>[2x]MDYKDDDDKHMSLVLNDLLICCRQLEHDRATERKKEVEKFKRLIRDPETIKHLDRHSDSKQGKYLNWDAVFRFLQKYIQKETECLRIAKPNVSASTQASRQKKMQEISSLVKYFIKCANRRAPRLKCQELLNYIMDTVKDSSNGAIYGADCSNILLKDILSVRKYWCEISQQQWLELFSVYFRLYLKPSQDVHRVLVARIIHAVTKGCCSQTDGLNSKFLDFFSKAIQCARQEKSSSGLNHILAALTIFLKTLAVNFRIRVCELGDEILPTLLYIWTQHRLNDSLKEVIIELFQLQIYIHHPKGAKTQEKGAYESTKWRSILYNLYDLLVNEISHIGSRGKYSSGFRNIAVKENLIELMADICHQVFNEDTRSLEISQSYTTTQRESSDYSVPCKRKKIELGWEVIKDHLQKSQNDFDLVPWLQIATQLISKYPASLPNCELSPLLMILSQLLPQQRHGERTPYVLRCLTEVALCQDKRSNLESSQKSDLLKLWNKIWCITFRGISSEQIQAENFGLLGAIIQGSLVEVDREFWKLFTGSACRPSCPAVCCLTLALTTSIVPGTVKMGIEQNMCEVNRSFSLKESIMKWLLFYQLEGDLENSTEVPPILHSNFPHLVLEKILVSLTMKNCKAAMNFFQSVPECEHHQKDKEELSFSEVEELFLQTTFDKMDFLTIVRECGIEKHQSSIGFSVHQNLKESLDRCLLGLSEQLLNNYSSEITNSETLVRCSRLLVGVLGCYCYMGVIAEEEAYKSELFQKAKSLMQCAGESITLFKNKTNEEFRIGSLRNMMQLCTRCLSNCTKKSPNKIASGFFLRLLTSKLMNDIADICKSLASFIKKPFDRGEVESMEDDTNGNLMEVEDQSSMNLFNDYPDSSVSDANEPGESQSTIGAINPLAEEYLSKQDLLFLDMLKFLCLCVTTAQTNTVSFRAADIRRKLLMLIDSSTLEPTKSLHLHMYLMLLKELPGEEYPLPMEDVLELLKPLSNVCSLYRRDQDVCKTILNHVLHVVKNLGQSNMDSENTRDAQGQFLTVIGAFWHLTKERKYIFSVRMALVNCLKTLLEADPYSKWAILNVMGKDFPVNEVFTQFLADNHHQVRMLAAESINRLFQDTKGDSSRLLKALPLKLQQTAFENAYLKAQEGMREMSHSAENPETLDEIYNRKSVLLTLIAVVLSCSPICEKQALFALCKSVKENGLEPHLVKKVLEKVSETFGYRRLEDFMASHLDYLVLEWLNLQDTEYNLSSFPFILLNYTNIEDFYRSCYKVLIPHLVIRSHFDEVKSIANQIQEDWKSLLTDCFPKILVNILPYFAYEGTRDSGMAQQRETATKVYDMLKSENLLGKQIDHLFISNLPEIVVELLMTLHEPANSSASQSTDLCDFSGDLDPAPNPPHFPSHVIKATFAYISNCHKTKLKSILEILSKSPDSYQKILLAICEQAAETNNVYKKHRILKIYHLFVSLLLKDIKSGLGGAWAFVLRDVIYTLIHYINQRPSCIMDVSLRSFSLCCDLLSQVCQTAVTYCKDALENHLHVIVGTLIPLVYEQVEVQKQVLDLLKYLVIDNKDNENLYITIKLLDPFPDHVVFKDLRITQQKIKYSRGPFSLLEEINHFLSVSVYDALPLTRLEGLKDLRRQLELHKDQMVDIMRASQDNPQDGIMVKLVVNLLQLSKMAINHTGEKEVLEAVGSCLGEVGPIDFSTIAIQHSKDASYTKALKLFEDKELQWTFIMLTYLNNTLVEDCVKVRSAAVTCLKNILATKTGHSFWEIYKMTTDPMLAYLQPFRTSRKKFLEVPRFDKENPFEGLDDINLWIPLSENHDIWIKTLTCAFLDSGGTKCEILQLLKPMCEVKTDFCQTVLPYLIHDILLQDTNESWRNLLSTHVQGFFTSCLRHFSQTSRSTTPANLDSESEHFFRCCLDKKSQRTMLAVVDYMRRQKRPSSGTIFNDAFWLDLNYLEVAKVAQSCAAHFTALLYAEIYADKKSM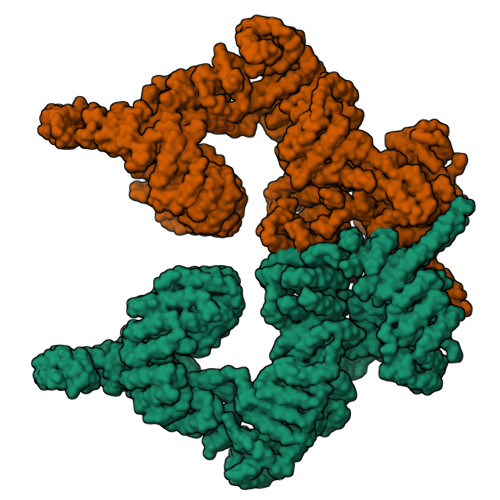DDQEKRSLAFEEGSQSTTISSLSEKSKEETGISLQDLLLEIYRSIGEPDSLYGCGGGKMLQPITRLRTYEHEAMWGKALVTYDLETAIPSSTRQAGIIQALQNLGLCHILSVYLKGLDYENKDWCPELEELHYQAAWRNMQWDHCTSVSKEVEGTSYHESLYNALQSLRDREFSTFYESLKYARVKEVEEMCKRSLESVYSLYPTLSRLQAIGELESIGELFSRSVTHRQLSEVYIKWQKHSQLLKDSDFSFQEPIMALRTVILEILMEKEMDNSQRECIKDILTKHLVELSILARTFKNTQLPERAIFQIKQYNSVSCGVSEWQLEEAQVFWAKKEQSLALSILKQMIKKLDASCAANNPSLKLTYTECLRVCGNWLAETCLENPAVIMQTYLEKAVEVAGNYDGESSDELRNGKMKAFLSLARFSDTQYQRIENYMKSSEFENKQALLKRAKEEVGLLREHKIQTNRYTVKVQRELELDELALRALKEDRKRFLCKAVENYINCLLSGEEHDMWVFRLCSLWLENSGVSEVNGMMKRDGMKIPTYKFLPLMYQLAARMGTKMMGGLGFHEVLNNLISRISMDHPHHTLFIILALANANRDEFLTKPEVARRSRITKNVPKQSSQLDEDRTEAANRIICTIRSRRPQMVRSVEALCDAYIILANLDATQWKTQRKGINIPADQPITKLKNLEDVVVPTMEIKVDHTGEYGNLVTIQSFKAEFRLAGGVNLPKIIDCVGSDGKERRQLVKGRDDLRQDAVMQQVFQMCNTLLQRNTETRKRKLTICTYKVVPLSQRSGVLEWCTGTVPIGEFLVNNEDGAHKRYRPNDFSAFQCQKKMMEVQKKSFEEKYEVFMDVCQNFQPVFRYFCMEKFLDPAIWFEKRLAYTRSVATSSIVGYILGLGDRHVQNILINEQSAELVHIDLGVAFEQGKILPTPETVPFRLTRDIVDGMGITGVEGVFRRCCEKTMEVMRNSQETLLTIVEVLLYDPLFDWTMNPLKALYLQQRPEDETELHPTLNADDQECKRNLSDIDQSFNKVAERVLMRLQEKLKGVEEGTVLSVGGQVNLLIQQAIDPKNLSRLFPGWKAWV> MNRHSAGQSTPVRVATLDQLKPGVPTAFDVDGDEVMVVRDGDSVYAISNLCSHAEAYLDMGVFHAESLEIECPLHVGRFDVR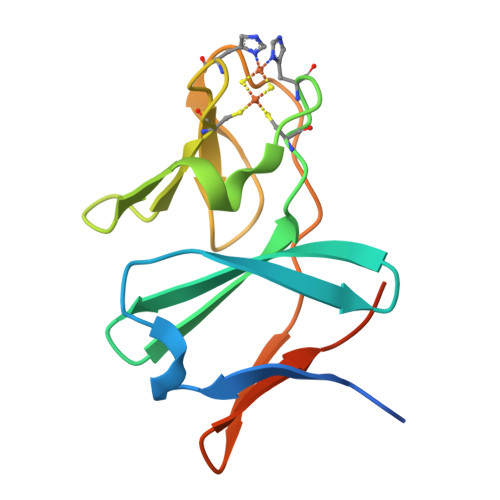TGAPTALPCVLPVRAYDVVVDGTEILVAPKEADHHHHHH>IEEVSNEEELKAALRDASITTIKLKNNITLNNAITINNGNRNITIIGDGHYINALNSDGGIILNNRGGSAKIDLTIENATLYNTSKYGFVNMSSNGVDTVTYKDVTAYGGTLVWSKTGAGVKTLNLVGNTTLNSVKSYEVDGQSCGTEAFSHRTPDGDKTTALYVSNAINI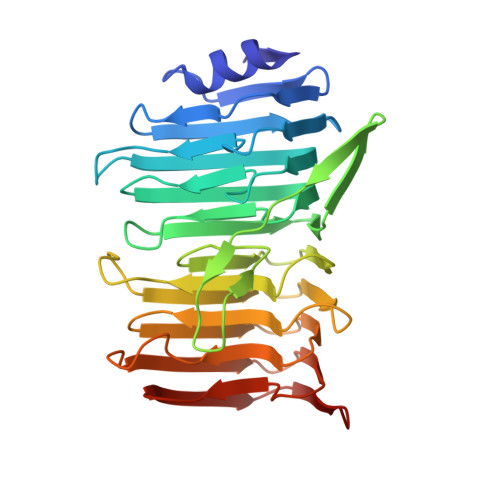AENANVVLNNSATDIDMWLLTAVPSTSGISTVTVGNNASLTMENIGNTEYNIKLDGGRENHFIVNENAAVKMSAKVDNVRIIPQLENIFTRGNIELAKGSNVHLEVITGSNFRVAGTVANRIDFNGTATLIKQEGASGP[3x]> LLAEPQIAMFCGRLNMHMNVQNGKWDS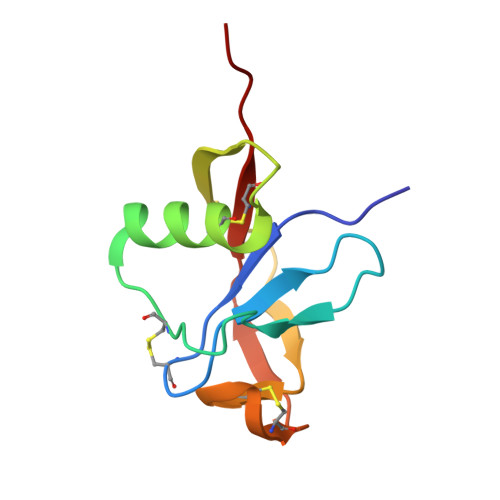DPSGTKTCIDTKEGILQYCQEVYPELQITNVVEANQPVTIQNWCKRGRKQCKTHPHFVIPYRCLVGEFV>ATCYC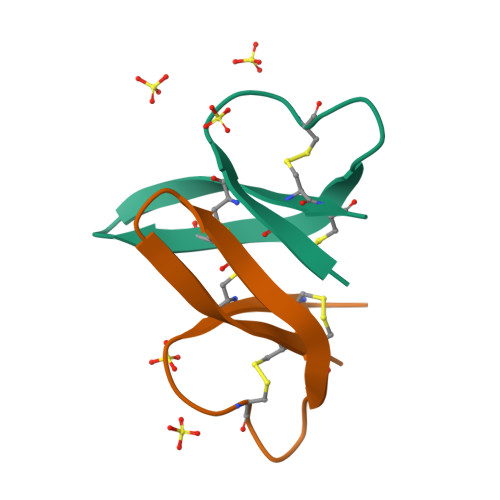RRGRCATRESLSGVCRISGRLYRLCCR[4x]> MEITTLQIVLVFIVACIAGMGSILDEFQFHRPLIACTLVGIVLGDMKTGIIIGGTLEMIALGWMNIGAAVAPDAALASIISTILVIAGHQSIGAGIALAIPLAAAGQVLTIIVRTITVAFQHAADKAADNGNLTAISWIHVSSLFLQAMRVAIPAVIVALSVGTSEVQNM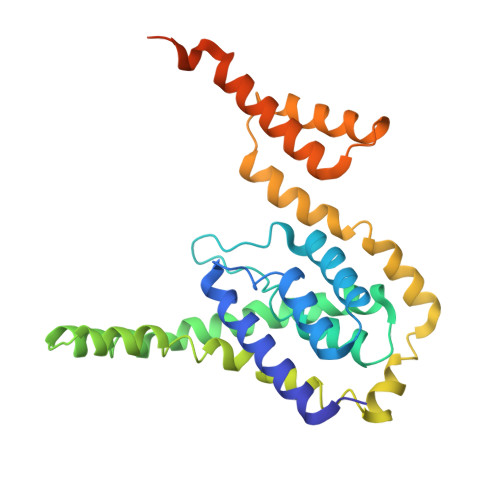LNAIPEVVTNGLNIAGGMIVVVGYAMVINMMRAGYLMPFFYLGFVTAAFTNFNLVALGVIGTVMAVLYIQLSPKYNRVAGAPAQAAGNNDLDNELDHHHHHHHH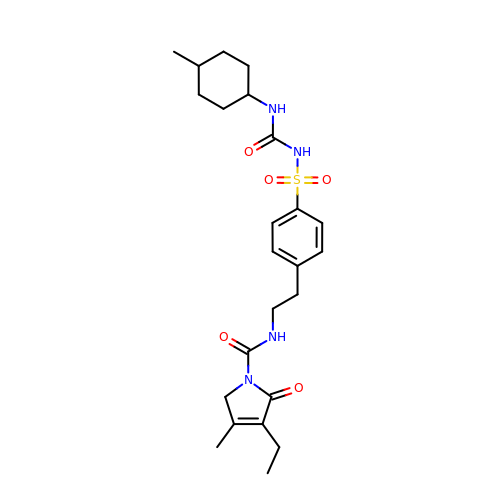3-ethyl-4-methyl-N-[2-(4-{[(cis-4-methylcyclohexyl)carbamoyl]sulfamoyl}phenyl)ethyl]-2-oxo-2,5-dihydro-1H-pyrrole-1-carboxamide | C24 H34 N4 O5 S | WIGIZIANZCJQQY-UWUNEBHHSA-N> MDGSGEQPRGGGPTSSEQIMKTGALLLQGFIQDRAGRMGGEAPELALDPVPQDASTKKLSESLKRIGDELDSNMELQRMIAAVDTDSPREVFFRVAADMFSDGNFNWGRVVALFYFASKL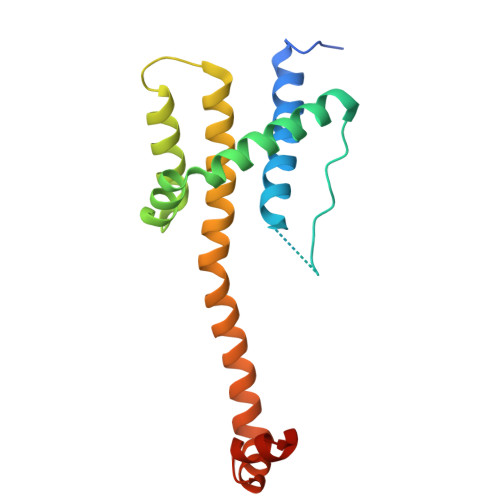VLKALSTKVPELIRTIMGWTLDFLRERLLGWIQDQGGWDGLLSYFGTPTW> TQWDDWVDKMENLNHDILTTLHT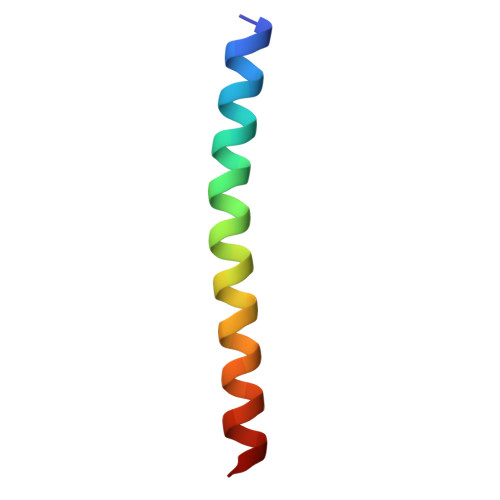ARNNLEQSMITFNT4-(cyclopentylmethylamino)-2-[[2-methoxy-4-(2-oxidanylidenepyrrolidin-1-yl)phenyl]amino]-7H-pyrrolo[2,3-d]pyrimidine-5-carbonitrile 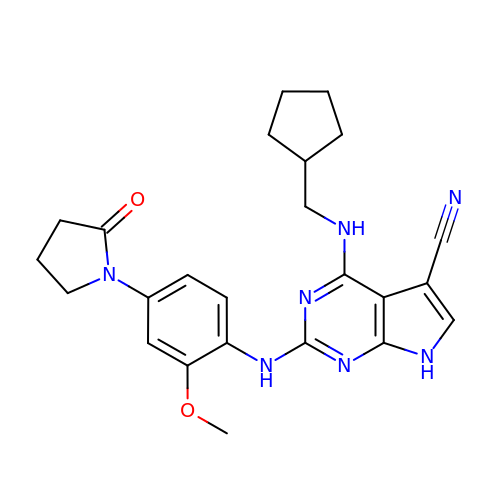| C24 H27 N7 O2 | HNTNJDLDWXMVRF-UHFFFAOYSA-N>[4x]MTSASSPPAFRLETSDGDEEGNAEVNKGKQEPPPMESPFQREDRNSSPQIKVNLNFIKRPPKNTSAPSQQEPDRFDRDRLFSVVSRGVPEELTGLLEYLRWNSKYLTDSAYTEGSTGKTCLMKAVLNLQDGVNACIMPLLQIDKDSGNPKPLVNAQCTDEFYQGHSALHIAIEKRSLQCVKLLVENGADVHLRACGRFFQKHQGTCFYFGELPLSLAACTKQWDVVTYLLENPHQPASLEATDSLGNTVLHALVMIADNSPENSALVIHMYDGLLQMGARLCPTVQLEEISNHQGLTPLKLAAKEGKIEIFRHILQREFSGPYQPLSRKFTEWCY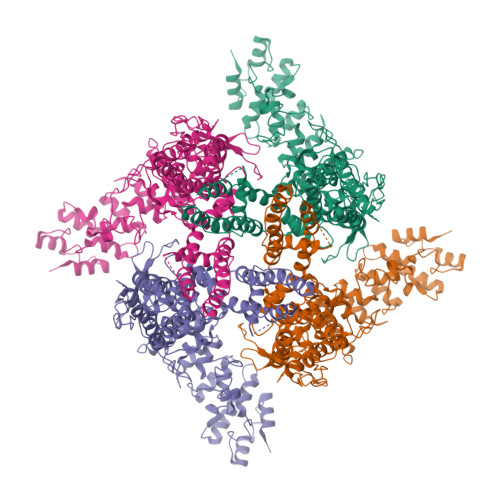GPVRVSLYDLSSVDSWEKNSVLEIIAFHCKSPNRHRMVVLEPLNKLLQEKWDRLVSRFFFNFACYLVYMFIFTVVAYHQPSLDQPAIPSSKATFGESMLLLGHILILLGGIYLLLGQLWYFWRRRLFIWISFMDSYFEILFLLQALLTVLSQVLRFMETEWYLPLLVLSLVLGWLNLLYYTRGFQHTGIYSVMIQKVILRDLLRFLLVYLVFLFGFAVALVSLSREARSPKAPEDNNSTVTEQPTVGQEEEPAPYRSILDASLELFKFTIGMGELAFQEQLRFRGVVLLLLLAYVLLTYVLLLNMLIALMSETVNHVADNSWSIWKLQKAISVLEMENGYWWCRRKKHREGRLLKVGTRGDGTPDERWCFRVEEVNWAAWEKTLPTLSEDPSGPGITGNKKNPTSKPGKNSASEEDHLPLQVLQSPTETSQVAPA> MRFKKHVVQHEETMQAIAQRYYGDVSYWIDLVEHNNLKYPYLVETDEEKMKDPERLASTGDTLIIPIESDLTDVSAKEINSRDKDVLVELALGRDLNITADEKYFNEHGTSDNILAFSTNGNGDLDTVKGIDNMKQQLQARLLTPRGSLMLHPNYGSDLHNLFGLNIPEQATLIEMEVLRTLTSDNRVKSANLIDWKIQGNVYSGQFSVEIKSVEESINFVLGQDEEGIFALFE;>MKTRKLTNILSKLIDKTMAGTSKITDFTPGSASRSLLEAVSLEIEQFYILTKENIDWGIQEGIIEAFDFQKRQSKRAYGDVTIQFYQPLDMRMYIPAGTTFTSTRQEYPQQFETLVDYYAEPDSTEIVVEVYCKETGVAGNVPEGTINTIASGSSLIRSVNNEYSFNTGTKEESQEDFKRRFHSFVESRGRATNKSVRYGALQIPDVEGVYVYEETGHITVFAHDRNGNLSDTLKEDIIDALQDYRPSGIMLDVTGVEKEEVNVSATVTISNKSRIGDTLQKHIESVIRSYLNNLKTSDDLIITDLIQAIMNIDDVLIYDVSFDNLDENIIVPPQGIIRAGEIKVELK[2x];> MANFLKNLHPLLRRDRNKKDNQDPNFALIDALNEEMNQVEKDAIESKLQSSLKTSTSEYLDKFGDWFGVYRKTDEKDDVYRARIIKYLLLKRGTNNAIIDAIKDYLGRDDIDVSVYEPFTNIFYTNKSHLNGEDHLMGYYYRFAVINVSIGDYFPVEIIDVINEFKPAGVTLYVTYDGASTIRGGAIIKWLDGLPKIETYQEFDRFTGYDDTFYGHINMNQSKDTDNSSSDIFKTNHSLINSLDVLTGSSSVGRQYINYGYVTSYVYNPGMTSSVNQISASTEGRGQEVPTDYYMYTSTKNNNTVELSMQTTSGVSYLYNNFNFRDYMSKYRPQVDLQSDEARRIVSDYIKELSIDYYLSAVIPPDESIEIKLQVYDFSINRWLTVSINNLSFYEKNIGSNIGYIKDYLNSELNMFTRLEINAGKRDSVDIKVNYLDLMFYYYERGIYTIKPYKALIENYLDISRETYVEAFKIASLSNGDIITKTGFQPIGYLKLVGNYENTIPSTINIVAKDTDNNPIESNELDVYNTVENRNLLQSYKGVNTIAREITSTKEFTVSGWAKEIYSTNYLSKVLKPGKVYTLSFDMEITGNDPTLKSYSDNHGIYLYSNTKGIVVNGVKSMERTIGNKVSVTQTFTAPTITDHRLLIYTGRYTSDGKASTPPVFFNTVKITELKLTEGSSKLEYSPAPEDKPNVIEKGIKFNNILTNIQTLSINSDTILKNVTLYYSYYGDSWVELKTLGNISTGETTETNNLIDLYGLQTVDYSNINPMSKVSLRSIWNVKLGELNNQEGSLSNMPNDYFNAVWQDIDKLSDIELGSMRMVKDTEGGVFDGATGEIIKATLFNVGAYTDLDMLAYTLTNYTEPLTLGSSRLISELKEELLTSESFNVDNRIKVIDSIYEELPNTSIIKNGFVEREVTGSKYLDYGLYEPIEDGTRYKLIVEGEFKDNIEFISLYNSNPNFNETFIYPSEIINGVAEKEFIAKPSTEDKPRLNTDVRIYIRPYDSTISKVRRVELRKV;>[3x]MAINFKGSPYLDRFDPSKDRTKVLFNPDRPLQQAELNEMQSIDQYYLKNLGDAIFKDGDKQSGLGFTLSEDNVLTVNPGYVYINGKIRYYDNDDSVKITGVGKETIGIKLTERIVTPDEDASLLDQTSGVPSYFSKGADRLEEKMSLTVNDPTSATIYTFMDGDLYIQSTNAEMDKINKVLAERTYDESGSYKVNGFELFSEGNAEDDDHVSVVVDAGKAYVKGFKVDKPVSTRISVPKSYDLGTAENESTIFNKSNNSISLANSPVKEIRRVTGQVLIEKERVTRGAQGDGQDFLSNNTAFEIVKVWTETSPGVTTKEYKQGEDFRLTDGQTIDWSPQGQEPSGGTSYYVSYKYNKRMEAGKDYEVTTQGEGLSKKWYINFTPSNGAKPIDQTVVLVDYTYYLARKDSVFINKYGDIAILPGEPNIMRLVTPPLNTDPENLQLGTVTVLPDSDEAVCISFAITRLSMEDLQKVKTRVDNLEYNQAVNALDDGAMEGQNPLTLRSVFSEGFISLDKADITHPDFGIVFSFEDAEATLAYTEAVNQPKIIPGDTTAHIWGRLISAPFTEERTIYQGQASETLNVNPYNIPNKQGVLKLTPSEDNWIDTENVTITEQKTKKVTMKRFWRHNESYYGETEHYLYSNLQLDAGQKWKGETYAYDREHGRTGTLLESGGQRTLEEMIEFIRIRDVSFEVKGLNPNDNNLYLLFDGVRCAITPATGYRKGSEDGTIMTDAKGTAKGKFTIPAGIRCGNREVTLKNANSTSATTYTAQGRKKTAQDIIIRTRVTVNLVDPLAQSFQYDENRTISSLGLYFASKGDKQSNVVIQIRGMGDQGYPNKTIYAETVMNADDIKVSNNASAETRVYFDDPMMAEGGKEYAIVIITENSDYTMWVGTRTKPKIDKPNEVISGNPYLQGVLFSSSNASTWTPHQNSDLKFGIYTSKFNETATIEFEPIKDVSADRIVLMSTYLTPERTGCTWEMKLILDDMASSTTFDQLKWEPIGNYQDLDVLGLARQVKLRATFESNRYISPLMSSSDLTFTTFLTELTGSYVGRAIDMTEAPYNTVRFSYEAFLPKGTKVVPKYSADDGKTWKTFTKSPTTTRANNEFTRYVIDEKVKSSGTNTKLQVRLDLSTENSFLRPRVRRLMVTTRDE;> MAIATYNSHVELAKYLVSKADSVYLTIGKSTPWSNETNPPQPDENATVLQEVIGYKKATKVTLVRPSKSPEDDNKNLISYGNKSWVEVTPENAKAEGAKWVYLESSIVGDELPLGTYRQVGFVMDLVAKSGISKFNLVPSEVESTGTLLFFDNKQFQNRSEQTTAKERFIVEVDPNSSSVDKLAAALEHHHHHH;>[6x]MAVEPFPRRPITRPHASIEVDTSGIGGSAGSSEKVFCLIGQAEGGEPNTVYELRNYSQAKRLFRSGELLDAIELAWGSNPNYTAGRILAMRIEDAKPASAEIGGLKITSKIYGNVANNIQVGLEKNTLSDSLRLRVIFQDDRFNEVYDNIGNIFTIKYKGEEANATFSVEHDEET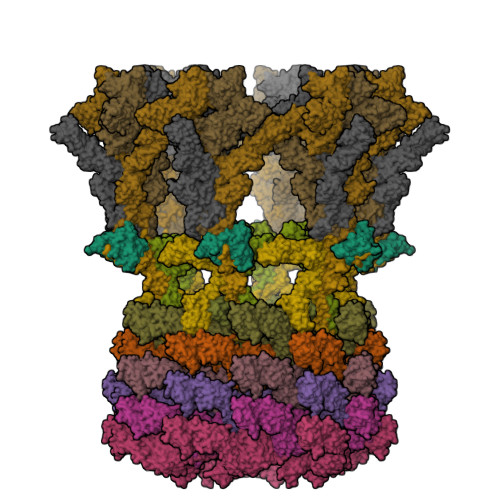QKASRLVLKVGDQEVKSYDLTGGAYDYTNAIITDINQLPDFEAKLSPFGDKNLESSKLDKIENANIKDKAVYVKAVFGDLEKQTAYNGIVSFEQLNAEGEVPSNVEVEAGEESATVTATSPIKTIEPFELTKLKGGTNGEPPATWADKLDKFAHEGGYYIVPLSSKQSVHAEVASFVKERSDAGEPMRAIVGGGFNESKEQLFGRQASLSNPRVSLVANSGTFVMDDGRKNHVPAYMVAVALGGLASGLEIGESITFKPLRVSSLDQIYESIDLDELNENGIISIEFVRNRTNTFFRIVDDVTTFNDKSDPVKAEMAVGEANDFLVSELKVQLEDQFIGTRTINTSASIIKDFIQSYLGRKKRDNEIQDFPAEDVQVIVEGNEARISMTVYPIRSFKKISVSLVYKQQTLQA> PPAVPQTFQVAHLHAPTGSGKSTKVPAAYAAQGYKVLVLNPSVAATLGFGVYMSKAHGIDPNIRTGVRAITTGGPITYSTYGKFLADGGCSGGAYDIIICDECHSTDSTSILGIGTVLDQAETAGARLVVLATATPPGSVTVPHPNIEEVALSNTGEIPFYGKAIPIEVIRGGRHLIFCHSKKKCDELAAKLSALGLNAVAYYRGLDVSVIPTSGDVVVVATDALMTGYTGDFDSVIDCNTCVTQTVDFSLDPTFTIDTTTVPQDAVSRSQRRGRTGRGRRGIYRFVTPGERPSGMFDSSVLCECYDAGCAWYELTPAETSVRLRAYLNTPGLPVCQDHLEFWESVFTGLTHIDAHFLS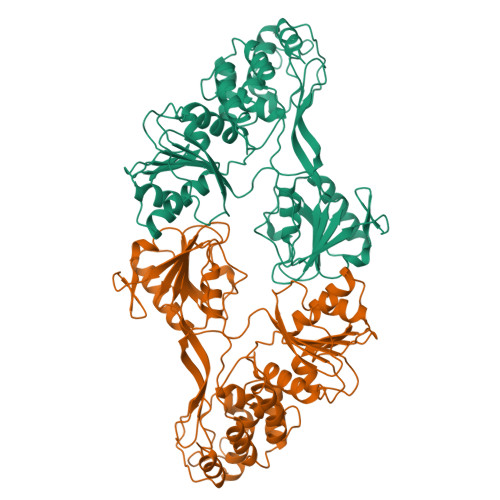QTKQAGDNFPYLVAYQATVCARAQAPPPSWDQMWKSLTRLKPTLHGPTPLLYRLGALQNEVTLTHPVTKFIMACMS>[2x]MAHHHHHHMKKNIFHNVSLYEIIFSDNGNTLTLSFTDTIEGNYFG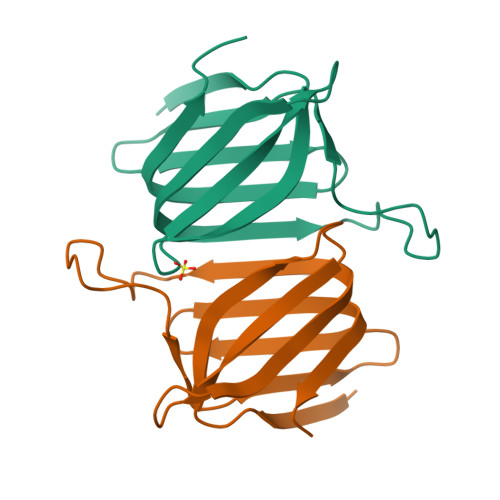YIKCSNILNFKLDTNNFVDYEDKEDSLFPLFIPEIELYKYQFYSEIIIDVGIIIKISAETINFEPLGK>APMMADRAKLLTTPGVFGNFSTYKVRADYMKLPAAERKAAAAEAQMVIDKHKDKVIVDTYLTRGLGAGSDYLLRVHSTDMAATQAFLVDWRATKLGMYSDVTENLVGITKALNYISKDKSPDLNAGLSSATYSDSAPRYVIVIPVKKDAAWWNMSDEQRLKEIEVHTQPTLQYLVN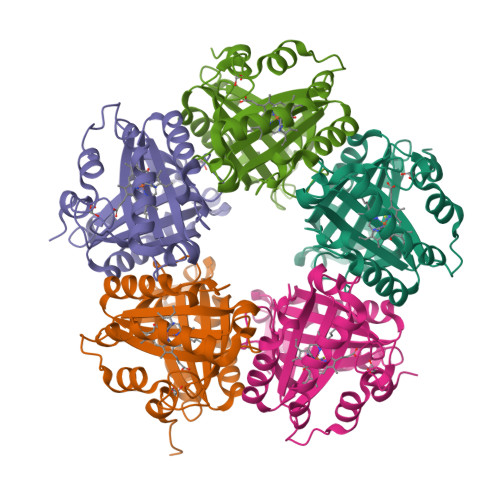VKRKLYHSTGLADADFITYFETADLAAFNNLLIALAKVPENTHHVRWGNPTVLGTIQSADVLVKTLSGM[10x]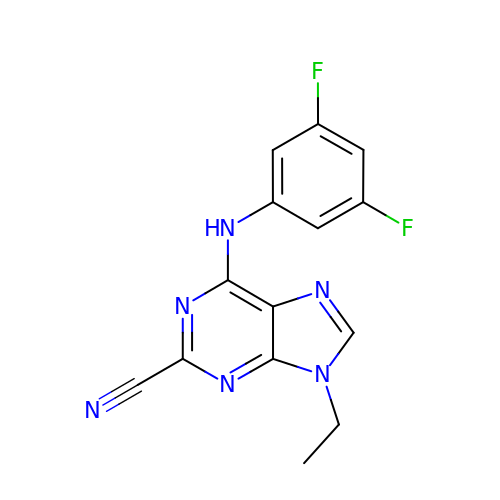6-[(3,5-difluorophenyl)amino]-9-ethyl-9H-purine-2-carbonitrile | C14 H10 F2 N6 | SZYYBVWPURUFRR-UHFFFAOYSA-N> DNTVQFDPF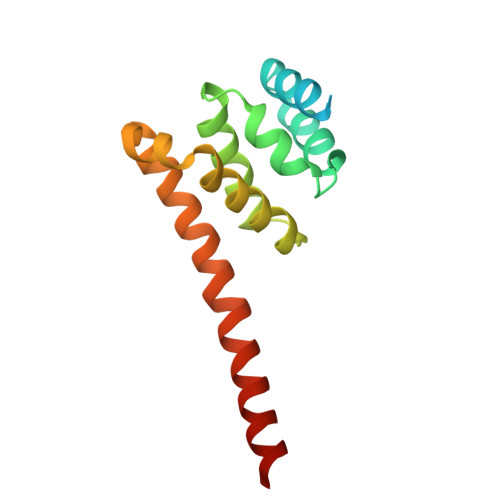DLNMEITPASTLAVLEKEKDYLKALVMAFRLNEAGLITRVYQAIPYTDIGLVVEQFPTVYVPRLLRFVAAQTEQSPHMEFCLLWIRALIDKHGPWLAANRGKVDVELRVVARAVAKMRDEIRRLADENVYMVDYLLNQAK> MKTLVHVASVEKGRSYEDFQKVYNAIALKLREDDEYDNAIGYGPVLVRLAWHTSGTWDKHDNTGGSYGGTYRFK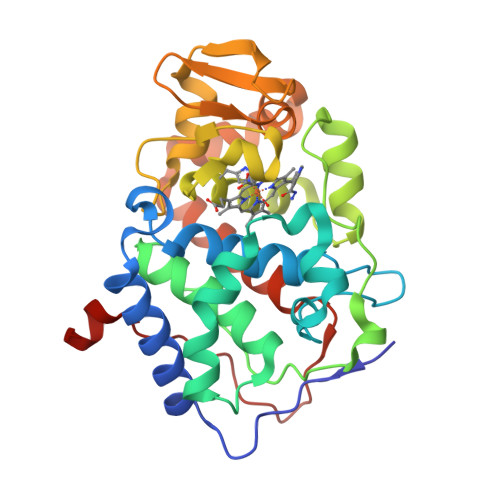KEFNDPSNAGLQNGFKFLEPIHKEFPWISSGDLFSLGGVTAVQEMQGPKIPWRCGRVDTPEDTTPDNGRLPDADKDADYVRTFFQRLNMNDREVVALMGAHALGKTHLKRSGYEGPWGAANNVFTNEFYLNLLNENWKLEKNDANNEQWDSKSGYMMLPTDYSLIQDPKYLSIVKEYANDQDKFFKDFSKAFEKLLENGITFPKDAPSPFIFKTLEEQGL1-(piperidin-4-ylmethyl)-1H-pyrazolo[3,4-d]pyrimidin-4-amine 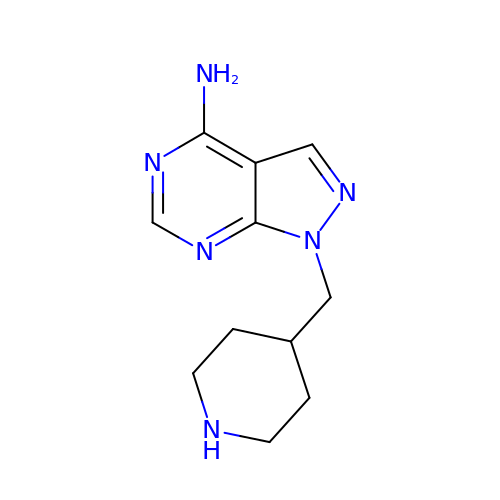| C11 H16 N6 | WIWYTHZSXOQVGK-UHFFFAOYSA-N>[2x]GPHMDLRPVVIDGSNVAMSHGNKEVFSCRGILLAVNWFL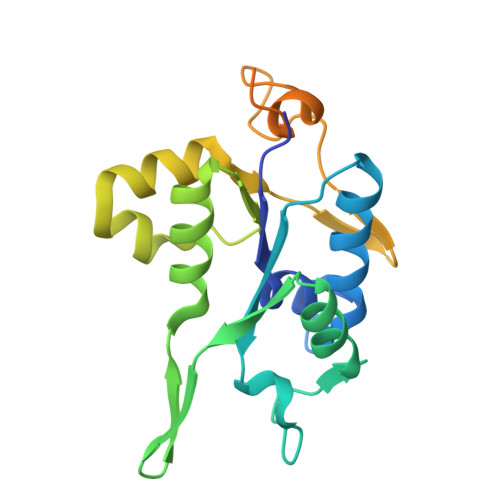ERGHTDITVFVPSWRKEQPRPDVPITDQHILRELEKKKILVFTPSRRVGGKRVVCYDDRFIVKLAFESDGVVVSNDTYRDLQGERQEWKRFIEERLLMYSFVNDKFMPPDDPLGRHGPSLDNFLRKKPLPSEHRKQPCPYGKKCTYGIKCRFFHPERPSRPQRSVADELRA> FQSMSVRPPVLVDIKFNPEGVDRVLKTAFADRGSINLADPANRERDFSETEYALLWKPDADLFRRAPNLKVIFSGGAGVDHIIGMAGLPDIPIVRFVDRSLTTRMSEWVVMQCLMHLRGQYGHDSHQRRREWAKLIAPEAAEVTVGVMGLGILGQDAVAKLKVMGFNVIGWSRTRKTIEGVETFDAGELDRFLAKTDILVGLLPLTPETTGFYDSELFKKLRRDGALGQPVFINAGRGKSQIETDIVSAVREGTLGGASLDVFEVEPLATDSPLWELENVFITPHDAAVSEENALFRHVEMQIARFERGEPLQFVIDR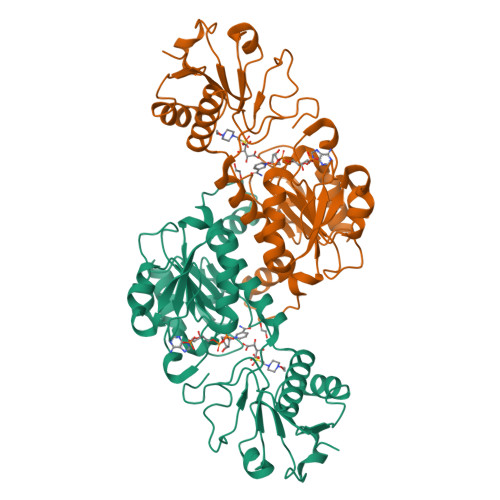AAGY4-(7-AMINO-9-HYDROXY-1-OXO-3,3A,4,5-TETRAHYDRO-2,5,6,8,9B-PENTAAZA-CYCLOPENTA[A]NAPHTHALEN-2-YL)-PHENYLCARBONYL-GLUTAMIC ACID | C20 H21 N7 O7 | 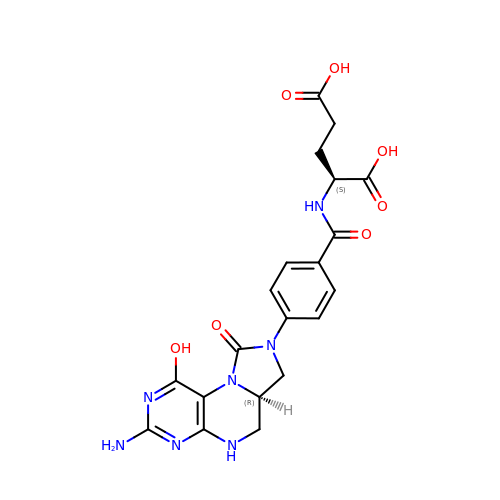JSNFRYBHBVDHSG-NEPJUHHUSA-N> MRLFVSD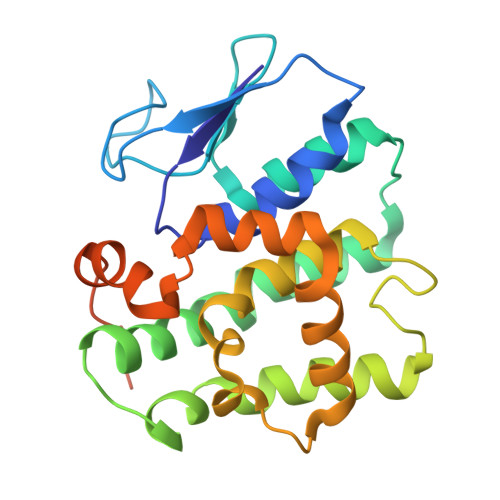GVPGCLPVLAAAGRARGRAEVLISTVGPEDCVVPFLTRPKVPVLQLDSGNYLFSTSAICRYFFLLSGWEQDDLTNQWLEWEATELQPALSAALYYLVVQGKKGEDVLGSVRRALTHIDHSLSRQNCPFLAGETESLADIVLWGALYPLLQDPAYLPEELSALHRWFQTLSTQEPCQRAAETVLKQQGVLALRPYLQKQPQPSPAEGRAVTNEPEEEELEHHHHHH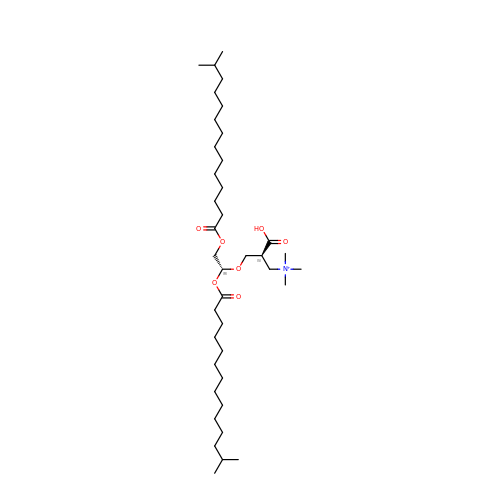[(2~{S})-2-[[(1~{R})-1,2-bis(13-methyltetradecanoyloxy)ethoxy]methyl]-3-oxidanyl-3-oxidanylidene-propyl]-trimethyl-azanium | C39 H76 N O7 | HRFZWHLOBWLUBX-ZGAWMTGXSA-O5-[(3aS,4S,6aR)-1,3-dimethyl-2-oxohexahydro-1H-thieno[3,4-d]imidazol-4-yl]pentanoic acid | C12 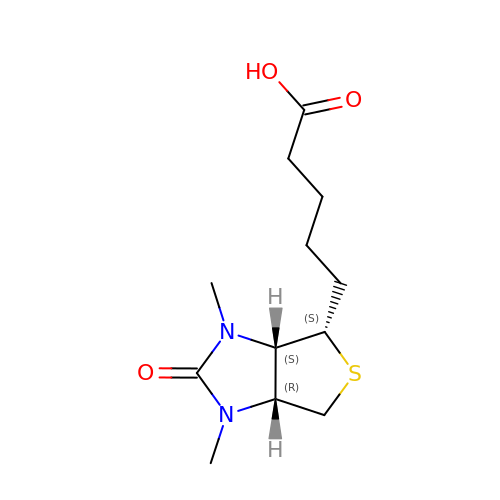H20 N2 O3 S | PECDAVNFXWSGFV-QXEWZRGKSA-N> MIHLRPDSTAYARSAAVSANPAVGGYVTPDNTVLEGQNPSALVQAMQKPVASVTDSFKATLSESIGAKALRGVEYASIPTEAGFEPSKALGDSVSQYTADELEFLSDARSSAELAQRRSQVQDTRNNYDAMGQNMLTTVAASMLDVDMVIGGGVGALSKVSRATRLAVGLSANAALLGTASYGGTITPLDVVGTSVGIAMSAIPGIRKVAKAEQVQQGAVRGGVNAAEDAAGTVVPPKDVTVPPVREVPEVQPI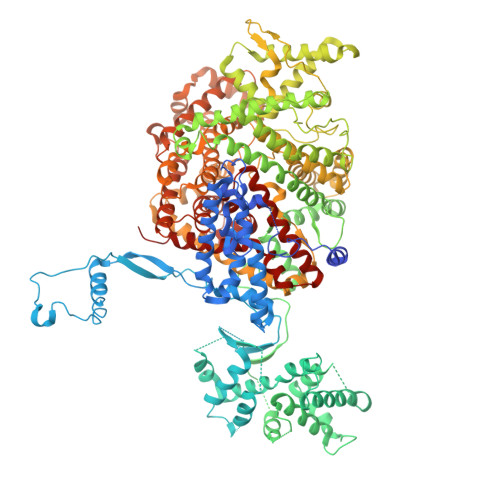KTVADEDYPKIDIDTYSNKEHIEVGRTGGAKTGSLKTTVQNAVLAVTALGDDLPEGVRALGRALGASLEADADVPVVFRSRTGANAQARSAVITEAETGATRAEIFNPAVGGTLSDHVRGMSTYEKTILLHEAAHAKTGRSIRAVESGAVSDGVVYEAVQRIKEIQWYVKANVELPPLGKGAKYNVDYGLSDTHEFISQLFNSEHFRDALRSVKMPGSDGTLLSNLMKRVVTLFTGKAPEGNAFDATLQAFDNLLSQPTTPADVFLNAPKATPDLQSKVLQAPNVIEMNNKVMGALNRNFSLYERLKSFGYKASTLADQLVVDATGTEANSAAHHARAAHLASNVSIVQVDDAFRQALSADWPLVQRLRHPVLYREAQRDLSQKVYQQLAENHDRFLKGQSIQPSNDPRVNSMVDAFVNSNWAKDELARVKGAGINGADAVRESPYYLPRQHSGNKLNDFMRNNRQVTKDDIVGMYTEQFSRMFQQNGITPETARKLGAKMFDNMQDQAAHVQGYRQSIAGMSYDDIENTLEALGASDPTITAFLDAVKGSGEQANKVRNLRGRAEFDMTAQYTTKSGDMISPSMFVNNDVMGLMEGYSRRMSGRVGLAKAGFPDLRDAVKAIDEAAAEAQDPAAALHAFDNTMNQILGYPTGEDVPDILRSASIIGGALNLANSGIYQLADMSLMLQQFGITKTLKAFGSTAFGRNAMDVAKSAEFGSRLQDVIEARHVLSGKYRSVLTHLEDNRDIGSLGVAHRYVQQMGQGTRFVNGMEFIRRGQAKLVSGLIADTVDDAIAGNASAVTAMERFGLNQQLLDELRKATAANPDMRKWPDSVRMDIEAVTHNMADSIVLENRLGEIPAWMQFSSVGKVILPYMTFVAGAWNKILRRTAKLDGATGVAIALAYQMPLVTLSSATSIAISGKPVTPESVAQRALVQVPMMSWAGFAVDFWANGASNNLAALALVDRMHAAMSSIASGETNPESLIKAVPFLSILPGMRLMGASLADDDE> EETEEQINARLTKLVNAAPVMLFMKGSPSEPKCGFSRQLVGILREHQVRFGFFDILRDESVRQNLKKFSEWPTFPQLYINGEFQGG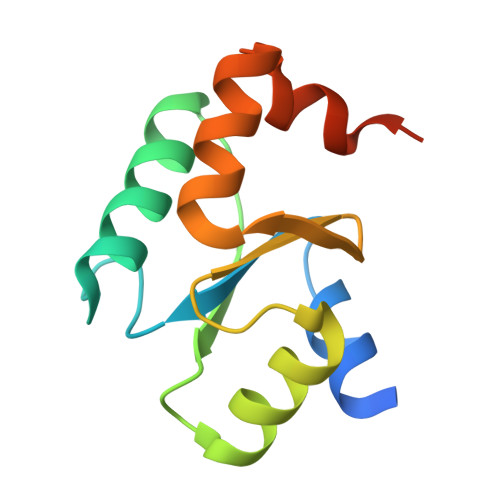LDIIKESLEEDPDFLQHALQSLEHHHHHH Escherichia coli NfsB has been studied extensively for its potential for cancer gene therapy by reducing the prodrug CB1954 to a cytotoxic derivative. The natural substrate of this flavoprotein enzyme is not known; however, it reduces a wide range of nitroaromatic compounds to hydroxylamines and also reduces quinones to quinols, with a bi-bi substituted (ping-pong) enzyme mechanism. The enzyme is a homodimer of two 24 kDa subunits with an extensive dimer interface. The two active sites are on opposite sides of the long central helix at the dimer interface, and the FMN is bound to residues from both monomers.

The most active double mutant was T41L/N71S, where at position 41 the threonine is replaced by leucine, and at position 71 the asparagine is replaced by serine. The double T41L/N71S mutant combines the effects of two single mutations determined previously. On replacing N71 with S71, in most of the structures of all the mutants, a water-mediated hydrogen bond to the FMN cofactor is found from the Oγ of S71 instead of the direct hydrogen bond from the NH2 of N71. This water molecule also forms a hydrogen bond with K74, as does N71 NH2 in the wild-type enzyme. However, unlike N71, the S71 does not form a hydrogen bond with FMN O4. The leucine side chain at position 41 is larger than the native threonine. The longer side chain of the leucine causes slight shifts in the positions of F124 and W138, each of which is in van der Waals contact with one of the methyl groups of L41. At T41, the T41L mutation in the double mutant shows the same effects as seen in the single T41L mutant and the T41L/N71S/F124W mutant studied by Bai et al.. The T41L/N71S and T41Q/N71S/F124T mutants both have a slightly lower redox potential than the wild-type protein. This is most likely due to the N71S mutation, where a direct hydrogen bond to the FMN cofactor is replaced by a water-mediated bond.

>[2x]MDIISVALKRHSTKAFDASKKLTPEQAEQIKTLLQYSPSSLNSQPWHFIVASTEEGKARVAKSAAGNYVFSERKMLDASHVVVFCAKTAMDDVWLKLVVDQEDADGRFATPEAKAANDKGRKFFADMHRKDLHDDAEWMAKQVYLNVGNFLLGVAALGLDAVPIEGFDAAILDAEFGLKEKGYTSLVVVPVGHHSVEDFNATLPKSRLPQNITLTEV> MAKPLTDQEKRRQISIRGIVGVENVAELKKSFNRHLHFTLVKDRNVATTRDYYFAL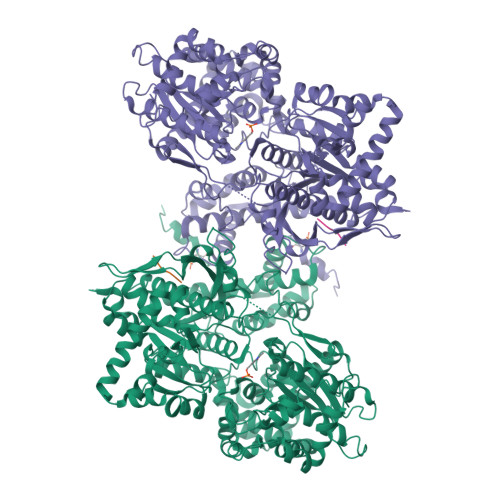AHTVRDHLVGRWIRTQQHYYDKCPKRVYYLSLEFYMGRTLQNTMINLGLQNACDEAIYQLGLDIEELEEIEEDAGLGNGGLGRLAACFLDSMATLGLAAYGYGIRYEYGIFNQKIRDGWQVEEADDWLRYGNPWEKSRPEFMLPVHFYGKVEHTNTGTKWIDTQVVLALPYDTPVPGYMNNTVNTMRLWSARAPNDFNLRDFNVGDYIQAVLDRNLAENISRVLYPNDNFFEGKELRLKQEYFVVAATLQDIIRRFKASKFGSTRGAGTVFDAFPDQVAIQLNDTHPALAIPELMRIFVDIEKLPWSKAWELTQKTFAYTNHTVLPEALERWPVDLVEKLLPRHLEIIYEINQKHLDRIVALFPKDVDRLRRMSLIEEEGSKRINMAHLCIVGSHAVNGVAKIHSDIVKTKVFKDFSELEPDKFQNKTNGITPRRWLLLCNPGLAELIAEKIGEDYVKDLSQLTKLHSFLGDDVFLRELAKVKQENKLKFSQFLETEYKVKINPSSMFDVQVKRIHEYKRQLLNCLHVITMYNRIKKDPKKLFVPRTVIIGGKAAPGYHMAKMIIKLITSVADVVNNDPMVGSKLKVIFLENYRVSLAEKVIPATDLSEQISTAGTEASGTGNMKFMLNGALTIGTMDGANVEMAEEAGEENLFIFGMRIDDVAALDKKGYEAKEYYEALPELKLVIDQIDNGFFSPKQPDLFKDIINMLFYHDRFKVFADYEAYVKCQDKVSQLYMNPKAWNTMVLKNIAASGKFSSDRTIKEYAQNIWNVEPSDLKISLSNESNKVNGN;> GPYY>[5x]DPFTMLQIEFITDLGARVTVNVEHESRLLDVQRHYGRLGWTSGEIPSGGYQFPIENEADFDWS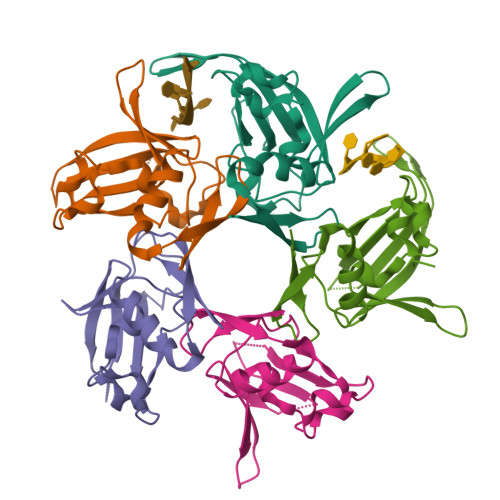LIGARKWKSPEGEELVIHRGHAYRRRELEAVDSRKLKLPAAIKYSRGAKVSDPQHVREKADGDIEYVSLAIFRGGKRQERYAVPG> MANKRMKVKHDDHYELIVDGRVYYICIVCKRSYVCLTSLRRHFNIHSWEKKYPCRYCEKVFPLAAYRTKHEIHHTGERRYQCLACGKSFINYQFMSSHIKSVHSQDPSGDSKLYRLHPCRSLQIRQ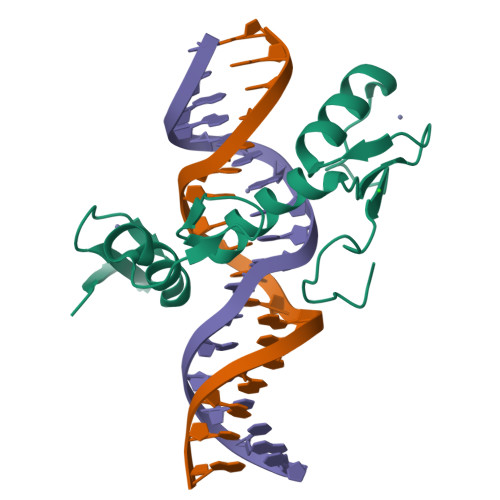YAYLSDRS1-(3-amino-2-methylbenzyl)-4-hexylpyridin-2(1H)-one | C19 H26 N2 O | 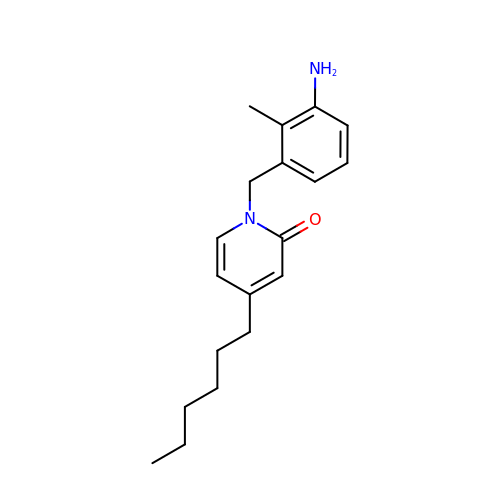PJADLCYVDLAZCT-UHFFFAOYSA-N>GPLGSPEFSPLLQPGLAELRRRVQEAGVPQTPQPLTDAFLLRFLRARDFDLDLAWRLMKNYYKWRAECPELSADLRPRSILGLLKAGYHGVLRSRDSTGSRVLIYRIAYWDPKVFTAYDVFRVSLITSELIVQEVETQRNGVKAIF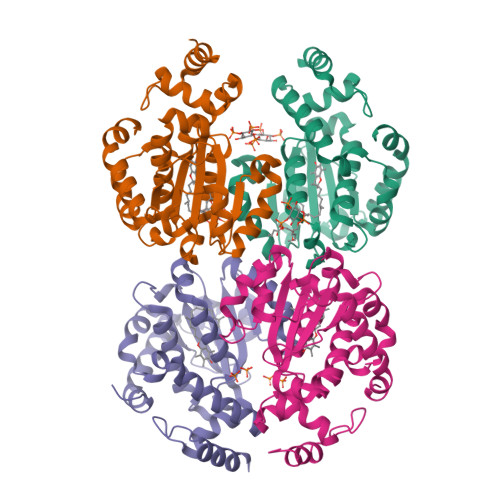DLEGWQVSHAFQITPSVAKKIAAVLTDSFPLKVRGIHLINEPVIFHAVFSMIKPFLTEKIKDRIHLHGNNYKSSMLQHFPDILPREYGGKEFSMEDICQEWTNFIMKSEDYLSSISETIQ[4x]> MAISRELVDPNSSPREIEVSEPREVGITELVLRDAHQSLMATRMAMEDMVGACADIDAAGYWSVECWGGTTYDSCIRFLNEDPWERLRTFRKLMPNSRLQMLLRGQNLLGYRHYNDEVVDRFVDKSAENGMDVFRVFDAMNDPRNMAHAMAAVKKAGKHAQGTICYTISPVHTVEGYVKLAGQLLDMGADSIALKDMAALLKPQPAYDIIKAIKDTYGQKTQINLHCHSTTGVTEVSLMKAIEAGVDVVDTAISSMSLGPGHNPTESVAEMLEGTGYTTNLDYDRLHKIRDHFKAIRPKYKKFESKTLVDTSIFKSQIPGGMLSNMESQLRAQGAEDKMDEVMAEVPRVRKAAGFPPLVTPSSQIVGTQAVFNVMMGEYKRMTGEFADIMLGYYGASP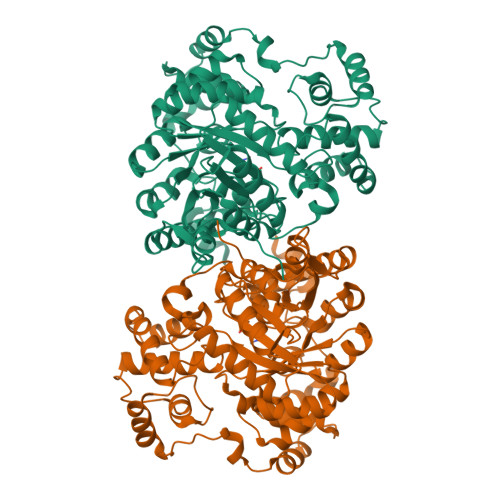ADRDPKVVKLAEEQSGKKPITQRPADLLPPEWEKQSKEAATLKGFNGTDEDVLTYALFPQVAPVFFEHRAEGPHSVALTDAQLKAEAEGDEKSLAVAGPVTYNVNVGGTVREVTVQQATRASQPELAPEDPEDLEHHHHHH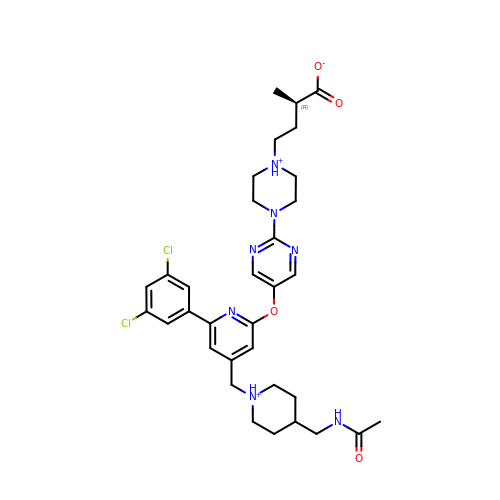(2R)-4-[4-[5-[4-[[4-(acetamidomethyl)piperidin-1-ium-1-yl]methyl]-6-[3,5-bis(chloranyl)phenyl]pyridin-2-yl]oxypyrimidin-2-yl]piperazin-1-ium-1-yl]-2-methyl-butanoate | C33 H42 Cl2 N7 O4 | GOXVJENOKGAJKU-JOCHJYFZSA-O>GSHMSYADSSRNAVLTNGGRTLRAECRNADGNWVTSELDLDTIIGNNDGHFQWGGQNFTETAEDIRFHPKEGAAEQPILRARL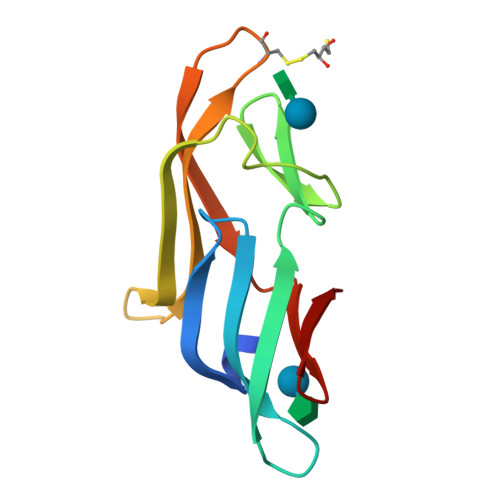RDCNGEFHDRDVNLNRIQNVNGRLVFQ[2x]>[4x]GPGSMARDATKLEATVAKLKKHWAESAPRDMRAAFSADPGRFGRYSLCLDDLLFDWSKCRVNDETMALLKELAVAADVEGRRAAMFAGEHINNTEDRAVLHVALRDTSSKEVLVDGHNVLPDVKHVLDRMAAFADGIRSGALKGATGRKITDIVNIGIGGSDLGPVMATLALAPYHDEPRAHFVSNIDGAHIA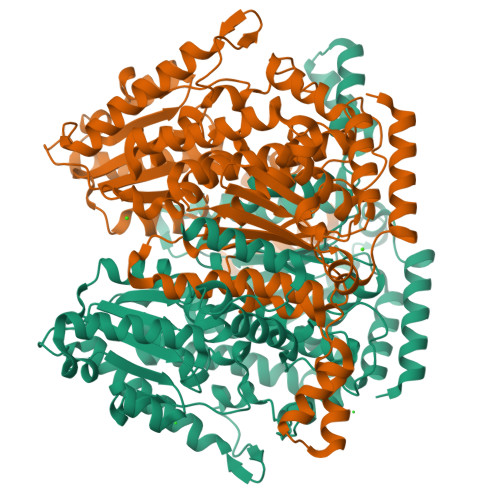DTLSPLDPASTLIIVASKTFTTIETMTNAQTARKWVADTLGEAAVGAHFAAVSTALDKVAAFGIPEDRVFGFWDWVGGRYSVWSAIGLPVMIAVGPDNFRKFLAGAHAMDVHFRDAPLEKNLPVMLGLIGYWHRAICGYGSRAIIPYDQRLSRLPAYLQQLDMESNGKSVTLDGKPVSGPTGPVVWGEPGTNGQHAFFQLLHQGTDTIPLEFIVAAKGHEPTLDHQHEMLMANCLAQSEALMKGRTLDEARAQLQAKNLPASQVERIAPHRVFSGNRPSLTLIHDMLDPYTLGRLIALYEHRVFVEAQIFGINAFDQWGVELGKELATELLPVVSGKEGASGRDASTQGLVAHLHARRKA>[2x]MSRLSEPSPYVEFDRRQWRALRMSTPLALTEEELVGLRGLGEQIDLLEVEEVYLPLARLIHLQVAARQRLFAATAEFLGEPQQNPDRPVPFIIGVAGSVAVGKSTTARVLQALLARWDHHPRVDLVTTDGFLYPNAELQRRNLMHRKGFPESYNRRALMRFVTSVKSGSDYACAPVYSH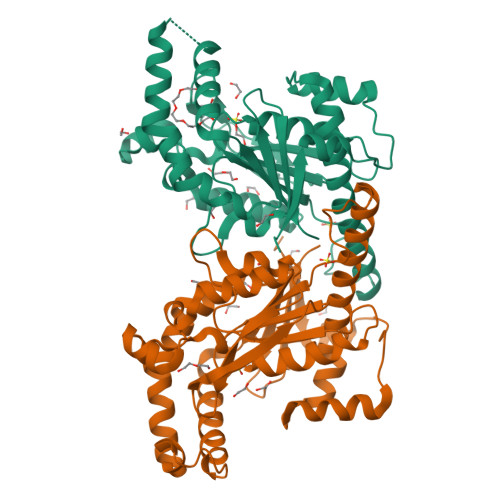LHYDIIPGAEQVVRHPDILILEGLNVLQTGPTLMVSDLFDFSLYVDARIEDIEQWYVSRFLAMRTTAAADPESHAHHYAAFSDSQAVVAAREIWRTINRPNLVENILPTRPRATLVLRKDADHSINRLRLRKL> CGTAC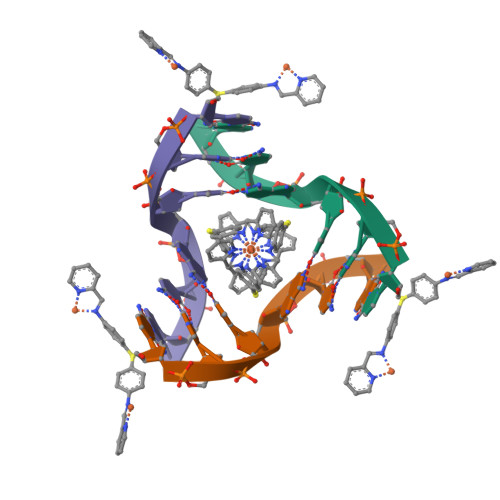G> MGSSHHHHHHSSGHIE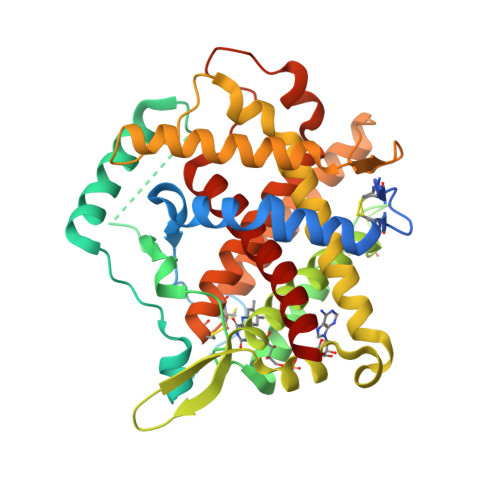GRHGEEQPPETAAQRCFCQVSGYLDDCTCDVETIDRFNNYRLFPRLQKLLESDYFRYYKVNLKRPCPFWNDISQCGRRDCAVKPAQSDEVPDGIKSASYKYSEEANNLIEEAEQAERLGAVDESLSEETQKAVLQWTKHDDSSDNFAEADDIQSPEAEYVDLLLNPERYTGYKGPDAWKIWNVIYEENCFKPQTIKRPLNPLASGQGTSEENTFYSWLEGLCVEKRAFYRLISGLHASINVHLSARYLLQETWLEKKWGHNITEFQQRFDGILTEGEGPRRLKNLYFLYLIELRALSKVLPFFERPDFQLFTGNKIQDEENKMLLLEILHEIKSFPLHFDENSFFAGDKKEAHKLKEDFRLHFRNISRIMDCVGCFKCRLWGKLQTQGLGTALKILFSEKLIANMPESGPSYEFHLTRQEIVSLFNAFGRISTSVKELENFRNLLQNIH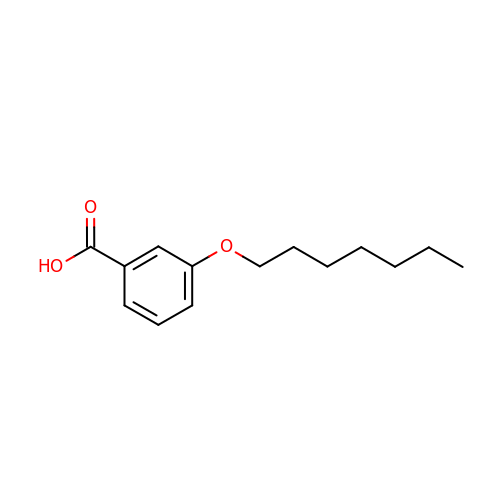3-(heptyloxy)benzoic acid | C14 H20 O3 | FOFZVIUYGPBWLV-UHFFFAOYSA-N5-(1-methylpyrazol-4-yl)-3-(3-propan-2-yloxyphenyl)furo[3,2-b]pyridine 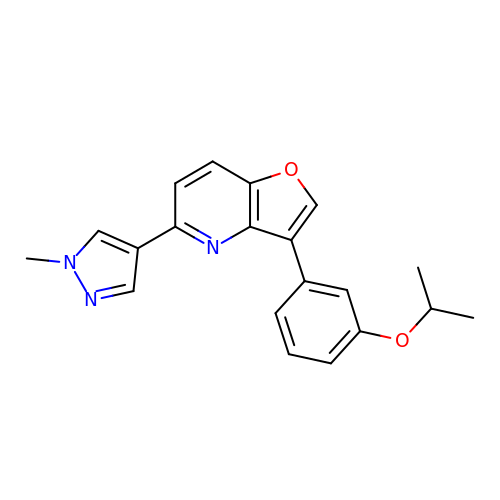| C20 H19 N3 O2 | QSJHQGFGDSZWSD-UHFFFAOYSA-N> MASDKFP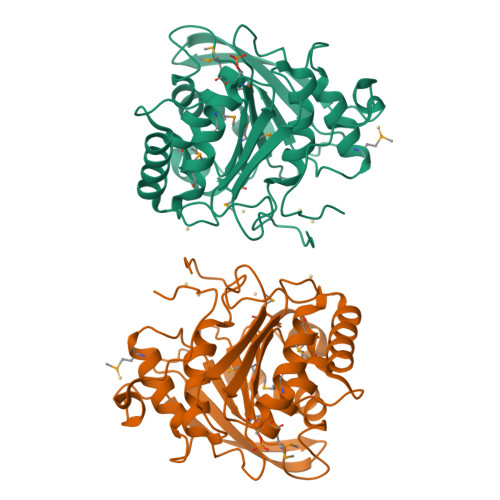VAENPSSSFKYESAVQYRPAPDSYLNPCPQAGRIVKETYTGINGTKSLNVYLPYGYDPNKKYNIFYLMHGGGENENTIFSNDVKLQNILDHAIMNGELEPLIVVTPTFNGGNCTAQNFYQEFRQNVIPFVESKYSTYAESTTPQGIAASRMHRGFGGFSMGGLTTWYVMVNCLDYVAYFMPLSGDYWYGNSPQDKANSIAEAINRSGLSKREYFVFAATGSEDIAYANMNPQIEAMKALPHFDYTSDFSKGNFYFLVAPGATHWWGYVRHYIYDALPYFFHELEHHHHHH> GPMTVFRQENVDDYYDTGEELGSGQFAVVKKCREKSTGLQYAAKFIKKRRTKSSRRGVSREDIEREVSILKEIQHPNVITLHEVYENKTDVILILELVAGGELFDFLAEKESLTEEEATEFLKQILNGVYYLHSLQIAHFDLKPENIMLLDRNVPKPRIKIIDFGLAHKIDFGNEFK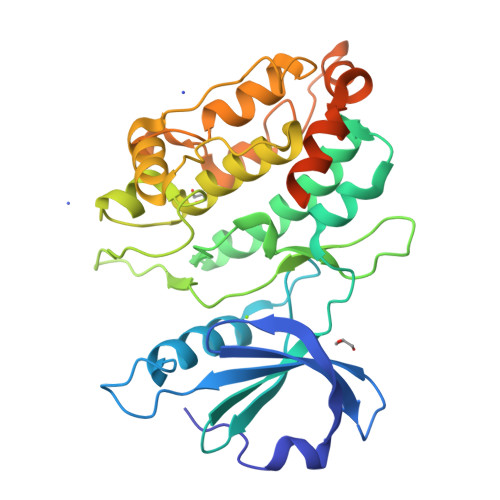NIFGTPEFVAPEIVNYEPLGLEADMWSIGVITYILLSGASPFLGDTKQETLANVSAVNYEFEDEYFSNTSALAKDFIRRLLVKDPKKRMTIQDSLQHPWIKPKDTQQALSRKAEAVNMEKFKKFAARKKWKQSVRLISLCQRLSRSFLSRSNMSVARSD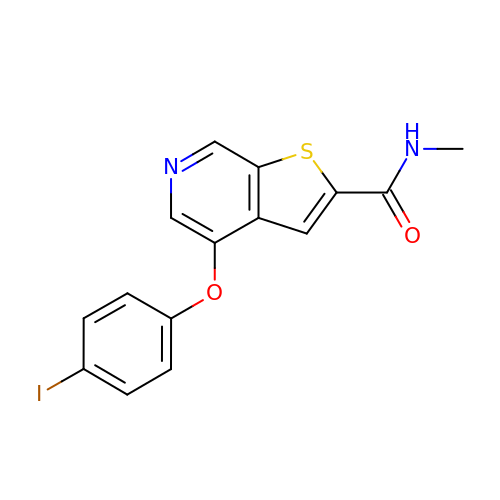4-(4-iodophenoxy)-N-methylthieno[2,3-c]pyridine-2-carboxamide | C15 H11 I N2 O2 S | QHMOZKVAGIEXJR-UHFFFAOYSA-N> MNEMFSQGGKGSTGILTNKQAIARHFGVKQSEVVYFSVGAVLSGYKVIYDKGTQRAYSLPANIGSGVTAISLSPAGVLVHSAGSVDLGALAVTRKEYVTLPDTFTSGSVIQTKNELLTHNGTQYRWAGGLPKSVPLNSTPVSAGGISPTAWVIANDELIRQELNNGLIPPVGSTSVYDVPGIVVNTTTDNRAAAYAFPGKIFIPNGVTIRCNLLPDDDVRKFVGEGKLIVKNQWYAKDHTFDIAASMNGNNKTVNDEIYCAFRDQTFCRIGIIGDSITDGAWGKQDWSSPPTNSDGDLDAPSTYNHSLSGGSHSWTEHWMNGLLLTQSRRSGETIYQSANCS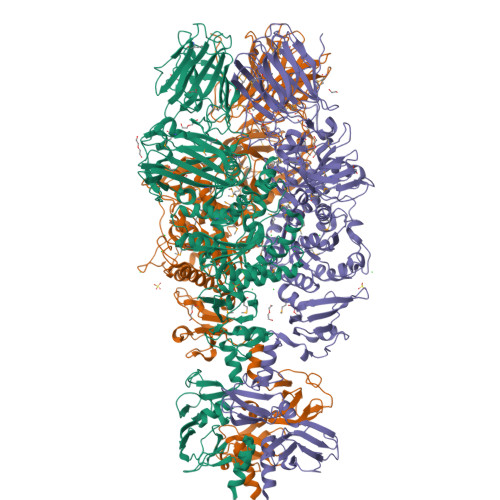VSGKKLSDGWGYRNFDRGFFGNTRYGAEAPRVCILAMGWNDSSASIATYRDQIDKFVRKAWGYGCAVGIVTVNDNDSVRMAFELSTKKYMADKLGVEYFNLGPNLTSASSRNEQTGYYYYVKKDGTWDTTHPQELGQMAMGNAMYMQTLGNKYCRRVRPGDMLTQAAVENYWDCVGYPSGTHYAPQYVPVSGAPALNVFRFLSKCVTNENVTMTTMVWCEEEGMTVSLLEPWTNAAVVGQSHNIRVESPVGKALFESGEYQERNTQINAYRTVLNGKTAMSYFGGGKTLTTYMGRLRKGLNFIRYIIDGSPTDAYFPMLKFGSYKTDGVKLPMVRLSKEPNMTRPAPVMKQSNANDYGVFGEVLSGTQFSKTADSHLYNGASVGYLAVPRGLKKNTYIALNYNPLTNVGVLVGVNAAGNMCIGTFNNANPTDWVVFGDTTREDKGFKVWEYTSSSTGAHTFTVESDDGTATTSAFSTTVATSGYVGLYNPSASSQLFTLEYSMTIGNVGLEHHHHHH N-(3-methoxyphenyl)-9H-purin-6-amine 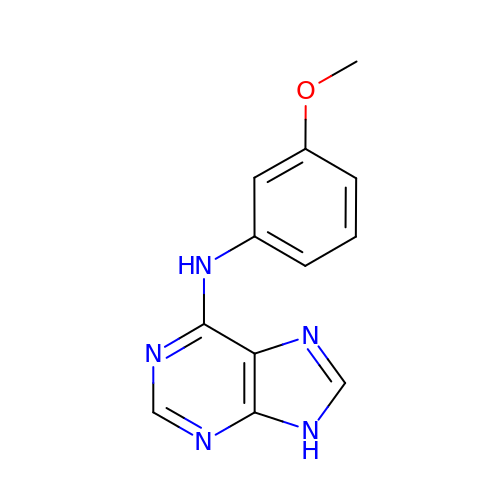| C12 H11 N5 O | AXPCHVXFDHPTBW-UHFFFAOYSA-N>LYDRRSIFDAVAQSNCQELESLLPFLQRSKKRLTDSEFKDPETGKTCLLKAMLNLHNGQNDTIALLLDVARKTDSLKQFVNASYTDSYYKGQTALHIAIERRNMTLVTLLVENGADVQAAANGDFFKKTKGRPGFYFGELPLSLAACTNQLAIVKFLLQNSWQPADISARDSVGNTVLHALVEVADNTVDNTKFVTSMYNEILILGAKLHPTLKLEEITNRKGLTPLALAASSGKIGVLAYILQREIHEPECRHLSRKFTEWAYGPVHSSLYDLSCIDTCEKNSVLEVIAYSSSETPNRHDMLLVEPLNRLLQDKWDR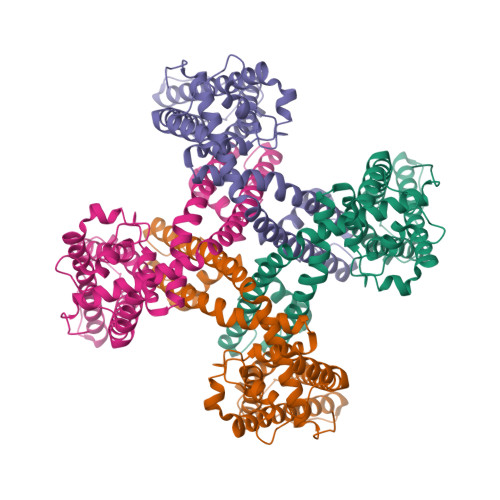FVKRIFYFNFFVYCLYMIIFTAAAYYRPVEGLPPYKLKNTVGDYFRVTGEILSVSGGVYFFFRGIQYFLQRRPSLKSLFVDSYSEILFFVQSLFMLVSVVLYFSQRKEYVASMVFSLAMGWTNMLYYTRGFQQMGIYAVMIEKMILRDLCRFMFVYLVFLFGFSTAVVTLIEDGKYNSLYSTCLELFKFTIGMGDLEFTENYDFKAVFIILLLAYVILTYILLLQMLIALMGETVNKIAQESKNIWKLQRAITILDTEKSFLKCMRKA[4x]SidN (Lpg1083) is one of the L. pneumophila T4SS effectors and does not exhibit sequence homology with any functionally annotated proteins. SidN, a hypothetical protein with unknown functions, is translocated into host cells in a Dot/Icm-dependent manner. Our results show that SidN is a nucleus-localized effector, and its structure adopts a novel fold. When ectopically expressed in mammalian cells, SidN is transported by Importin-13 into the nucleus, where it attaches to Lamin-B2 and interferes with structural integrity of the nuclear envelope architecture, leading to nuclear membrane disruption and eventually cell death.

In order to obtain clues about its function, we determined the crystal structure of SidN at 2.1 Å resolution by using the single-wavelength anomalous diffraction method. The SidN molecule forms a nearly cylindrical shape with a length of ∼60 Å and a diameter of ∼35 Å. The architecture folds into two domains. The smaller N-terminal paw-like domain (SidN1–82) is exclusively α-helical and formed by four helices (α1–α4). The larger C-terminal domain (SidN83–227) is composed of six α-helices (α5–α10), one 310 helix (η1), and a four-stranded anti-parallel β-sheet spatially arranged in the order β1/β2/β4/β3 from left to right when facing the sheet. Three anti-parallel helices (α5, α10, and α8) are packed against the β-sheet and the rest helices (α6, α7, α9, and η1). The two domains are connected by a very short loop. The C-terminal domain contacts the paw-like domain via the N-terminus of α6, as well as the loop between β2 and α6. However, the surface of SidN has a hydrophobic concave region lined with conserved residues on the end of the paw-like domain, suggesting that this region may serve as a binding hub. A single-amino acid change of phenylalanine (Phe19) or mutation of both phenylalanine (Phe19) and valine (Val40) in the center of the region to charged polar residues significantly decreased the punctate distribution of SidN at the ER and nuclear envelope, indicating that this conserved hydrophobic patch in the paw-like domain of SidN is essential for subcellular localization.

> MGHHHHHHMALIDQITTINKNEFTDDFLRKYFELGFGSLSKHDIDLLVYYLVKEHSDLFNGKTNYEISSLLTITERKLQSIQMESYLRYENNSISKNLEELSVKITKGEIKPEVEGDKIRVLIDSPVLRRDLEYSITSLGHIVDYSFNKNILSLRLSNFFEVFGNLNIENGKELKTQVIDFFREQNKWDKEILIEIENKSWWIKQFNTLQAAVKKEAAALIFHSIISMVKSHIGI(7alpha,8alpha,10alpha,13alpha)-7,16-dihydroxykauran-18-oic acid | C20 H32 O4 | 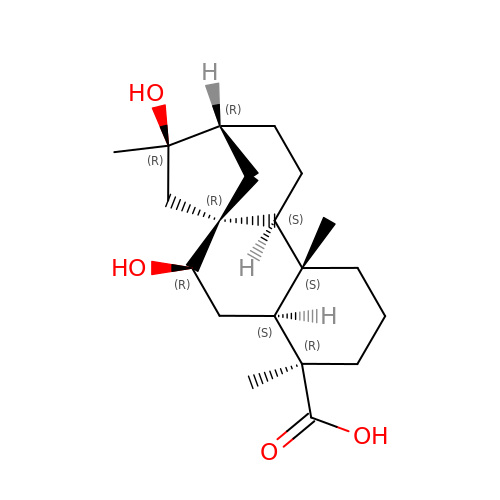HLTDMBIYZSPLMR-ONIYAHANSA-N>[4x]MAEYVFSDAPKDSHGNGVKDAVPGKQPEELPPAPRYFQGENTAGFMRPVRFEGDITNLEVVGEIPKSIEGTFYRVMPEPHLPSFIPNDPWFNGDGNISGFYFKDGHVDLKQRYVRTEKFVREAEARRSLLGKYRNRYTDLVEFKIRSTANTNIVYWRGQLLALKEDSPPYAMDPETLETFGVYDFDGQLPSLTFTAHPKFDPVTREMVCFGYEAKGDGTRDICYYSFGPDGKIAETVWLVSPVCGMIHDFAVTENFVIFPIIPLVCDVERMKQGGDHWQWDYSIPMYIGVLPRRGAQGSDVKWFEAPHGFAGHVANAFEDDKGHIQLQMAYAKDNVFFWWPDANGKGPRPGEVEAHFANFVLDYQSDKLPLAEPTYLVDDDMEFPRIDDRVATRKHKHTFFCIFDRKPGVTDFEFVMPRAGGG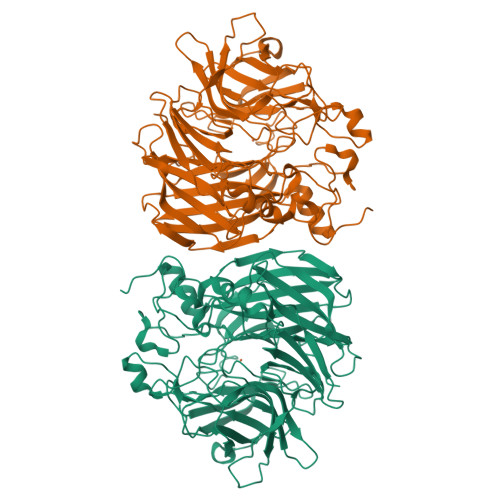APMSNGLAHLNHETGDIQRYLPGPRKLTGECIFIPRNSEAAEGDGYVMVLLANYEDMCSELAVLDTKDLTNEVALIKLPVRLRPGLHGNWVDKSDVDGHPAPL>AYDRAITVFSPDGRLFQVEYAREAVKKGSTALGMKFANGVLLISDKKVRSRLIEQNSIEKIQLIDDYVAAVTSGLVADARVLVDFARISAQQEKVTYGSLVNIENLVKRVADQMQQYTQYGGVRPYGVSLIFAGIDQIGPRLFDCDPAGTINEYKATAIGSGKDAVVSFLEREYKENLPEKEAVTLGIKALKSSLEEGEELKAPEIASITVGNKYRIYDQEEVKKFL[7x];>TTTVGITLKDAVIMATERRVTMENFIMHKNGKKLFQIDTYTGMTIAGLVGDAQVLVRYMKAELELYRLQRRVNMPIEAVATLLSNMLNQVKYMPYMVQLLVGGIDTAPHVFSIDAAGGSVEDIYASTGSGSPFVYGVLESQYSEKMTVDEGVDLVIRAISAAKQRDSASGGMIDVAVITRKDGYVQLPTDQIESRIRKLGLIL[7x];>[7x]KRAALIQNLRDSYTETSSFAVIEEWAAGTLQEIEGIAKAAAEAHGVIRNSTYGRAQAEKSPEQLLGVLQRYQDLCHNVYCQAETIRT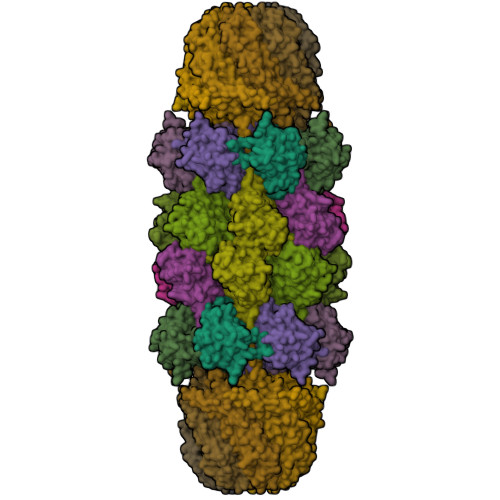VIAIRIPEHKEEDNLGVAVQHAVLKIIDELEIKTLGSGEKSGSGGAPTPIGMYALREYLSARSTVEDKLLGSVDAESGKTKGGSQSPSLLLELRQIDADFMLKVELATTHLSTMVRAVINAYLLNWKKLIQPRTHLDVLYR>[6x]GPGSMTDEILLSNTEERVRTLTLNRPQARNALSAALRDRFFGALADAETDDDVDVVIITGADPVFCAGLDLKELGGSSALPDISPRWPALTKPVIGAINGAAVTGGLELALYCDILIASENARFADTHARVGLLPTWGLSVRLPQKVGIGLARRMSLTGDYLSAADALRAGLVTEVVPHDQLLGAA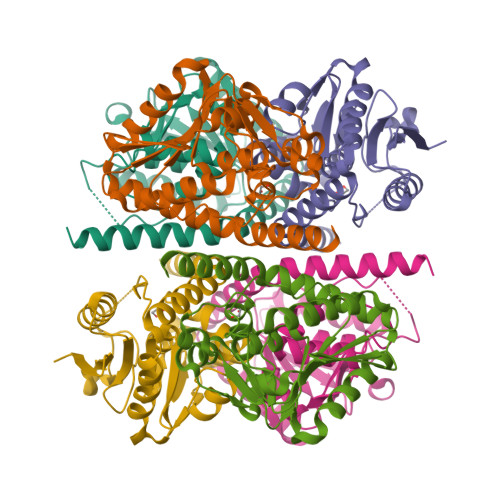QAVAASIVGNNQNAVRALLASYHRIDDAQTSAGLWQEAMAARQFRTSGDDIAANREAVLARGRSQVR> MAQASKGLIGALQASLGGLLSTSGRLHGGLGPSAGPAALVSGAWGLSACAAFTRSVATTSAGASATAPAEPGPASTASDAGSGAAQEAEAISSGSN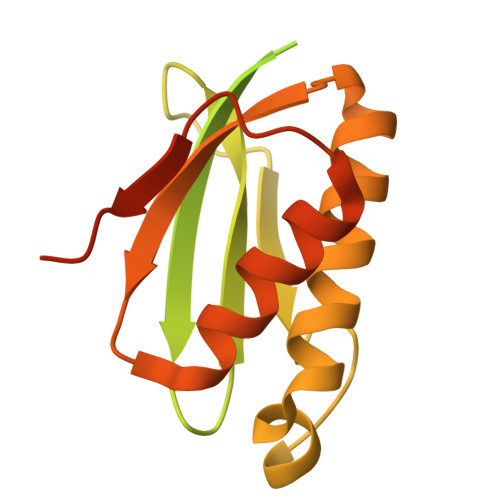SGGGGFSTGFRKVVSERRAGQLGALEGIVHIQNTLNNIILTLTDKQGLIKTYTSAGVVGYKGSRKSQPVAAEKAAEELARRALKLGYSSVQVRLKGAGSNKQYAVTSLAAAGLTITSLADVTPVPYNGCRLPKKRRV>[3x]TKKESFEDVLPSILNTITTNSELTEVPEVANWLKKVLEYNLAGGKKARGLTTLFAYEMLEKPENITEETIYLAKTLGWCVEILQGFLVMLDD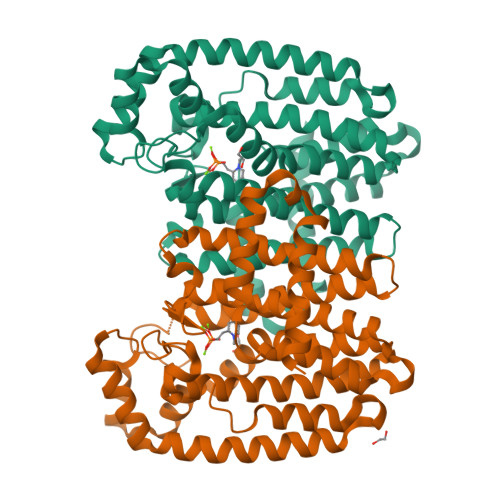IMDGSTTRRGVPCWYQLPEVGLAAVNDSSLMFSSIFYVLHAHFADKKIYTNLVELFNESLMHTSIGQHLDVTMERRQKSDYSLFTIERYNAIVKYKTAYYTYQLPVCLGMLLANISDPVLHQKAEDMCLEIGKFFQIQDDYIDCYGDESLTGKMGTDIQEAKCSWLAVMALQRCSASQKIVFTTCYGSKEPAHIERIKELYKQLQLPELYAQEETRMYESLIKQAHGLPSELSPALFVRLIHMIYKRNH>MGFLSGK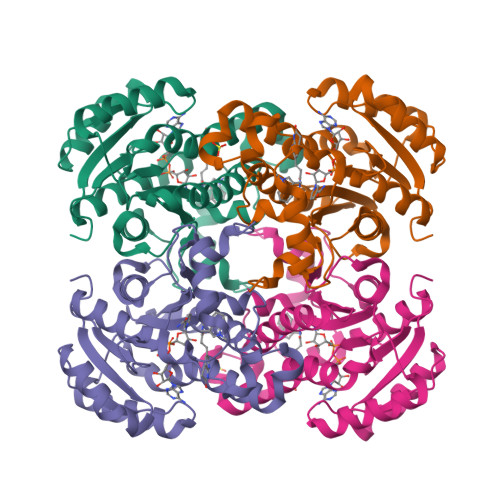RILVTGVASKLSIAYGIAQAMHREGAELAFTYQNDKLKGRVEEFAAQLGSDIVLQCDVAEDASIDTMFAELGKVWPKFDGFVHSIGFAPGDQLDGDYVNAVTREGFKIAHDISSYSFVAMAKACRSMLNPGSALLTLSYLGAERAIPNYNVMGLAKASLEANVRYMANAMGPEGVRVNAISAGPIRTLAASGIKDFRKMLAHCEAVTPIRRTVTIEDVGNSAAFLCSDLSAGISGEVVHVDGGFSIAAMNELELK[2x]2-fluoro-4-hydroxybenzonitrile | C7 H4 F N O | 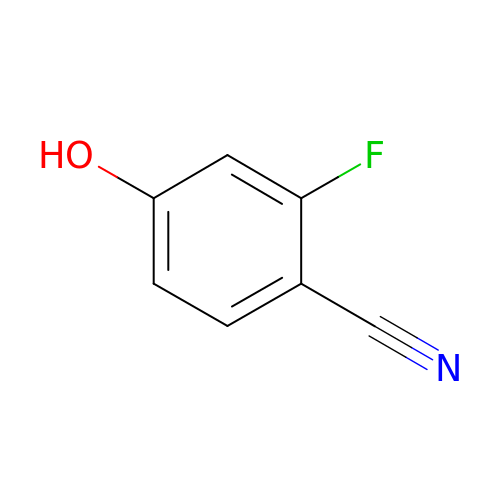REIVHYDACHXPNH-UHFFFAOYSA-N> IDYPSVSFNLAGAKSTTYRDFLKNLRDRVATGTYEVNGLPVLRRESEVQVKNRFVLVRLTNYNGDTVTSAVDVTNLYLVAFSANGNSYFFKDATELQKSNLFLGTTQHTLSFTGNYDNLETAAGTRRESIELGPNPLDGAITSLWYDGGVARSLLVLIQMVPEAARFRYIEQEVRRSLQQLTSFTPNALMLSMENNWSSMSLEVQLSGDNVSPFSGTVQLQNYDHTPRLVDNFEELYKITGIAILLFRCVATKT;> DGETCAIPAPFTRRIVGRDGLCVDVRNGYDTDGTPIQLWPCGTQRNQQWTFYNDKTIRSMGKCMTANGLNSGSYIMITDCSTAAEDATKWEVLIDGSIINPSSGLVMTAPSGASRTTLLLENNIHAASQGWTVSNDVQPIATLIVGYNEMCLQANGENNNVWMED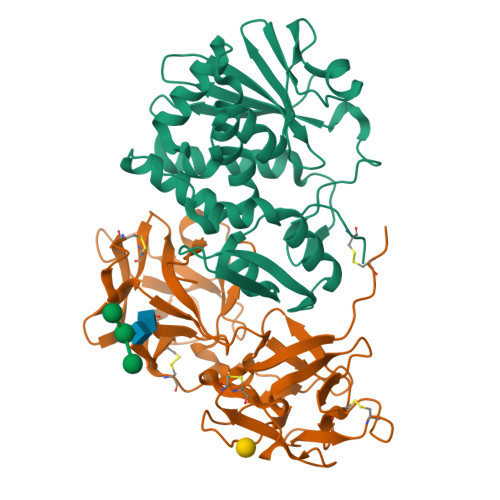CDVTSVQQQWALFDDRTIRVNNSRGLCVTSNGYVSKDLIVIRKCQGLATQRWFFNSDGSVVNLKSTRVMDVKESDVSLQEVIIFPATGNPNQQWRTQVPQI>MCSARSVRVVPRAATFEGLMDDASKAKMEELERRFKMADVDGNGHIDREELRNLLESMESGEVYMMSQHWLPEDELERCMEQYDVNKDGVISFEEFKQIIYDGLLLEGTLAEYESAFKAVDKSGNGTIGATELSKLFASLGNPVSLEKLVDLMQMYDKDDSGQIEFPEFLLMFRNSLLDLKDMTTYMTLDEAGAGSSGSLVDAVEGDMTLIFSEEELDALISANPDKLVVVFGALTWCRPCKGMQRPVQKLAEHYKDHIVFVKLFGNANKQTKRIFKERFQIRSTPCFITLRKGEPVYTQTGSNKEKLEAGLRSLIANPPV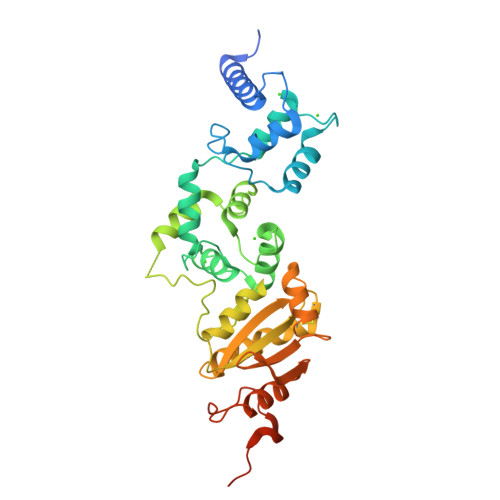GMIYPSAEALAALQDPNSSSVDKLAAALEHHHHHH[2x]>[2x]KEGYLVNKSTGC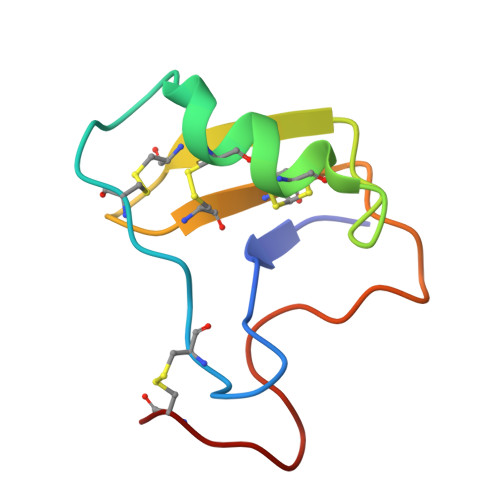KYGCLKLGENEGCDKECKAKNQGGSYGYCYAFACWCEGLPESTPTYPLPNKSCS> MEGAKPTLQLVYQAVQALYHDPDPSGKERASFWLGELQRSVHAWEISDQLLQIRQDVESCYFAAQTMKMKIQTSFYELPTDSHASLRDSLLTHIQNLKDLSPVIVTQLALAIADLALQMPSWKGCVQTLVEKYSNDVTSLPFLLEILTVLPEEVHSRSLRIGANRRTEIIEDLAFYSSTVVSLLMTCVEKAGTDEKMLMKVFRCLGSWFNLGVLDSNFMANNKLLALLFEVLQQDKTSSNLHEAASDCVCSALYAIENVETNLPLAMQLFQGVLTLETAYHMAVAREDLDKVLNYCRIFTELCETFLEKIVCTPGQGLGDLRTLELLLICAGHPQYEVVEISFNFWYRLGEHLYKTNDEVIHGIFKAYIQRLLHALARHCQLEPDHEGVPEETDDFGEFRMRVSDLVKDLIFLIGSMECFAQLYSTLKEGNPPWEVTEAVLFIMAAIAKSVDPENNPTLVEVLEGVVRLPETVHTAVRYTSIELVGEMSEVVDRNPQFLDPVLGYLMKGLAEKPLASAAAKAIHNICSVCRDHMAQHFNGLLEIARSLDSFLLSPEAAVGLLKGTALVLARLPLDKITECLSELCSVQVMALKKLLSQEPSNGISSDPTVFLDRLAVIFRHTNPIVENGQTHPCQKVIQEIWPVLSETLNKHRADNRIVERCCRCLRFAVRCVGKGSAALLQPLVTQMVNVYHVHQHSCFLYLGSILVDEYGMEEGCRQGLLDMLQALCIPTFQLLEQQNGLQNHPDTVDDLFRLATRFIQRSPVTLLRSQVVIPILQWAIASTTLDHRDANC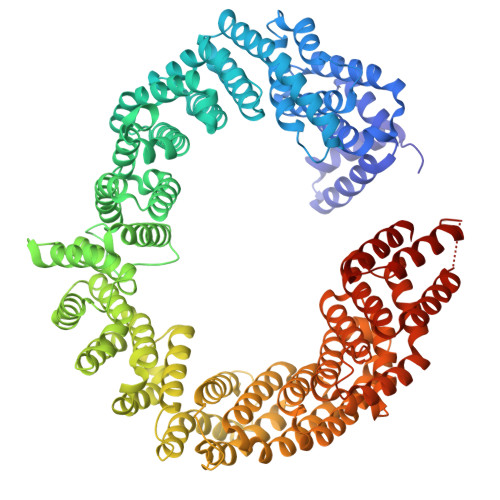SVMRFLRDLIHTGVANDHEEDFELRKELIGQVMNQLGQQLVSQLLHTCCFCLPPYTLPDVAEVLWEIMQVDRPTFCRWLENSLKGLPKETTVGAVTVTHKQLTDFHKQVTSAEECKQVCWALRDFTRLFR> MQRRQLLQSMGGLAASTMPFSL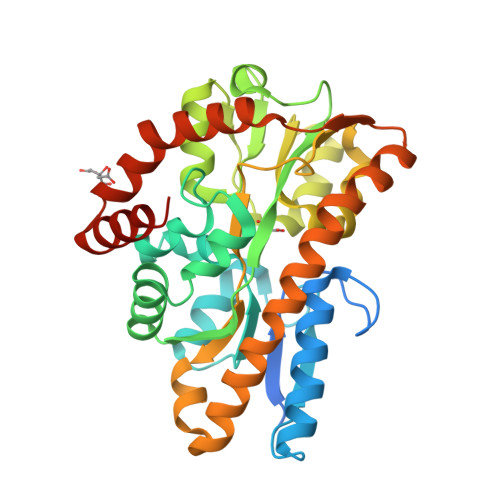AFAQTSALKISHQFPGGTIKEGDFRDRLVRNFAAEVEKRSKGAMKFEIYPGSSLMKTNAQFSSMRKGALDMALIPLSYAGGEVPELNIGLMPGLVVSYEQAYSWKTKPVGIELTRVLQEKGIVLISWIWQAGGVASRGKPVVEPEDAKGMKIRGGSREMDMILKDAGAAVVSLPSNEIYAAMQTGAMDAAMTSSTSFISFRLEEVAKALTTGRTGAYWFMFEPLMMSKAIFDKLPKDQRDMLMTVGAEMEKFALEAAKKDDIDVAAVYQKAGAKVVDLSDGTIKKWQDIARKTAWKDYGAKNEGCAKLLALAQQTLAENLYFQ> AESCTSRPHITVVEGEPFYLKHCSCSLAHEIETTTKSWYKSSGSQEHVELNPRSSSRIALHDCVLEFWPVELNDT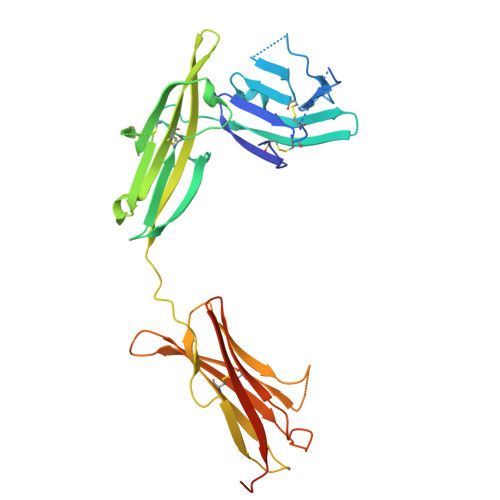GSYFFQMKNYTQKWKLNVIRRNKHSCFTERQVTSKIVEVKKFFQITCENSYYQTLVNSTSLYKNCKKLLLENNKNPTIKKNAEFEDQGYYSCVHFLHHNGKLFNITKTFNITIVEDRSNIVPVLLGPKLNHVAVELGKNVRLNCSALLNEEDVIYWMFGEENGSDPNIHEEKEMRIMTPEGKWHASKVLRIENIGESNLNVLYNCTVASTGGTDTKSFILVRKADMADIPGHVFTRHHHHHH biphenyl-4-yl 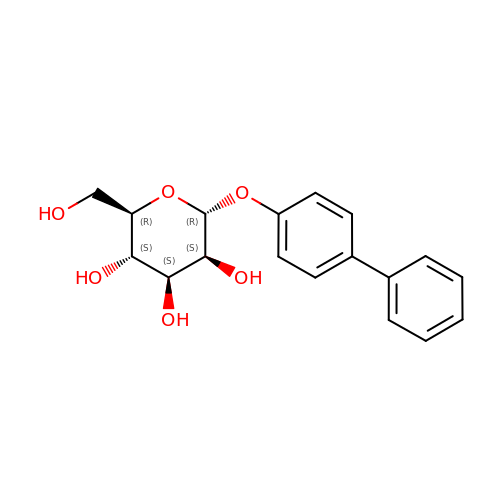alpha-D-mannopyranoside | C18 H20 O6 | SZBKRKVDBPBJHL-ZBRFXRBCSA-N>GPGGSGGMKPQIRNMVEPMDPRTFVSNFNNRPILSGLDTVWLCCEVKTKDPSGPPLDAKIFQGKVYPKAKYHPEMRFLRWFHKWRQLHHDQEYKVTWYVSWSPCTRCANSVATFLAKDPKVTLTIFVARLYYFWDPDYQQALRILAEAGATMKIMNYNEFQDCWNKFVDGRGKPFKPWNNLPKHYTLLQATLGELLRHLMDPGTFTSNFNNKPWVSGQHETYLCYKVERLHNDTWVPLNQHRGFLRNQAPNIHGFPKGRHAALCFLDLIPFWKLDGQQYRVTCFTSWSPCFSCAQEMAKFISNNEHVSLCIFAARIYDDQGRYQEGLRTLHRDGAKIAMMNYSEFEYCWDTFVDRQGRPFQPWDGL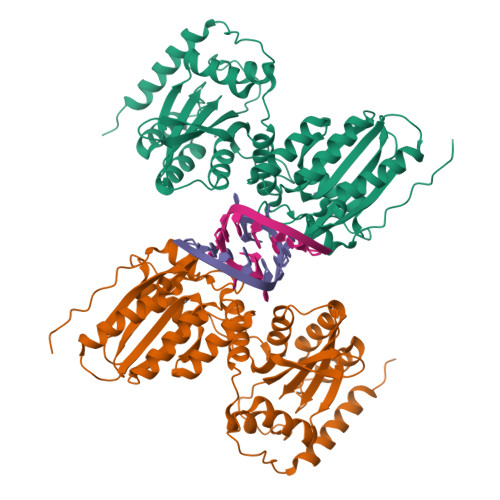DEHSQALSGRLRAILQNQGN[2x]>[3x]MRGSHHHHHHGSSAVSTTAAPEARSILAGAAEGKVIATTEALSFWGGVDPATGKVIDVHHPLHGICLTGGVLFMPTSRGSCTGSGVLLDLILTGRAPSALVFCEAEDVLTLGALVAAEMFDKALPVIRLDTETFARFSRAAHVRIDQNTIKADGVSLAVAPPATAHLDLTDDDRAMLEGRDGIAVRQAMRIIVAMAAQQGASALVDVTQGHIDGCIYASPANLTFAEKMADMGGKVRVPSTMNAISVDKANWRAQGVPEDFGDPAARLADAYVRMGCRPTFTCSPYLLDSAPSAGESIGWAESNAVIFANTVLGARTAKHPDFLDLCIAMTGRAPLSGVYLEENRRPQRIVDVALPAGIDDAFWPLVGYLAGKAVPDCIPLLRGLGAA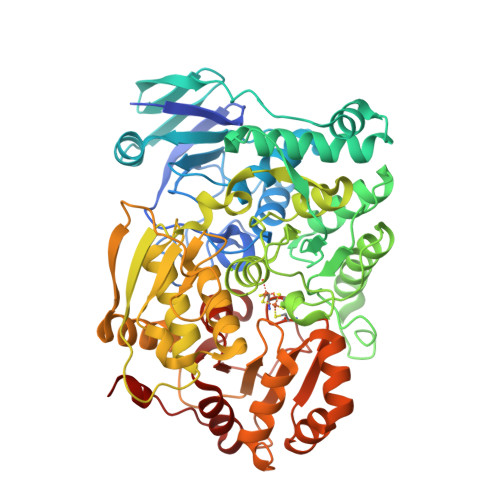KPSRDDLKALCAAFGTTSASPMLHIEGATPEAGLAPLETAETVTISLEDMAAGWSLLNEGPEEVQLVAIGSPHASLEECRALAAVFNGRKRHADVAVIVTAGQQVIDAAGKDGTLQSLKDSGVQVLPDLCWCSISEPVFPTKTRALMTNSGKYAHYGPGLSGRAVRFGSLADCVESALTGRAVSRLPVWLS>[3x]MKNKVVVVTGVPGVGSTTSSQLAMDNLRKEGVNYKMVSFGSVMFEVAKEENLVSDRDQMRKMDPETQK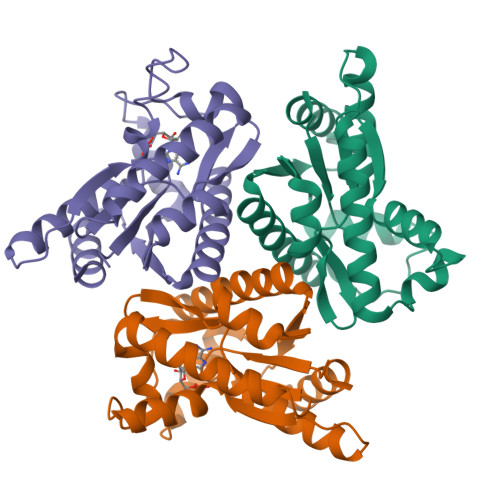RIQKMAGRKIAEMAKESPVAVDTHSTVSTPKGYLPGLPSWVLNELNPDLIIVVETTGDEILMRRMSDETRVRDLDTASTIEQHQFMNRCAAMSYGVLTGATVKIVQNRNGLLDQAVEELTNVLR>[2x]AFMALAYSNIPLGATVIPSPFQVHISDEQIEELQLLVKLSKLAPPTYEGLQQDRRY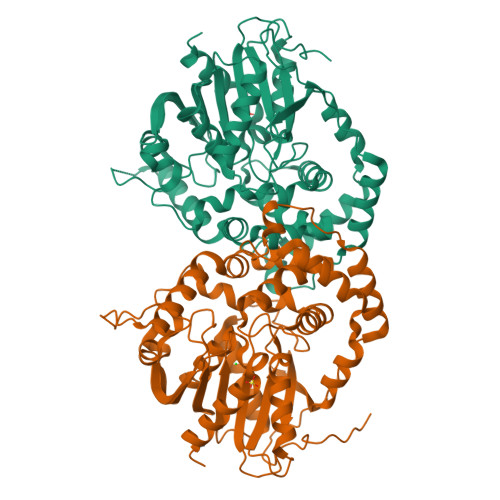GITNEWLANAKEAWKSFDWRPAESRINSFPQFTYDIEGLTIHFVALFSEKKDAIPIVLLHGWPGSFLEFLPVLTSIRDKYSPETLPYHIVVPSLPGYTFSSGPPLDVNFNGEDTARVINKVMLNLGFEDGYVAQGGDIGSKIGRILAVDHDACKAVHLNACYMGKPSSIPDTAITEEDKRALARAQWFATFGSGYAVEHGTRPSTIGNALSTSPVALLSWIGEKFLDWAGETIPLETILESVTLYWFTETFPRSIYHYRENFPPPKLRHTEDPRWYIRKPFGFSYYPMELVPTPRAWVETTGNLVFWQAHEKGGHFAALERPQDYLDDLTAFCEQVWAGRK>[12x]GPGSMTIIEVKIKKLENFLGNLPEYATEHSAGMDLVAANEQSITIKVGSIQLIPTGIAIALPESFEAQIRPRSGLAVKHGITVANSPGTIDADYRG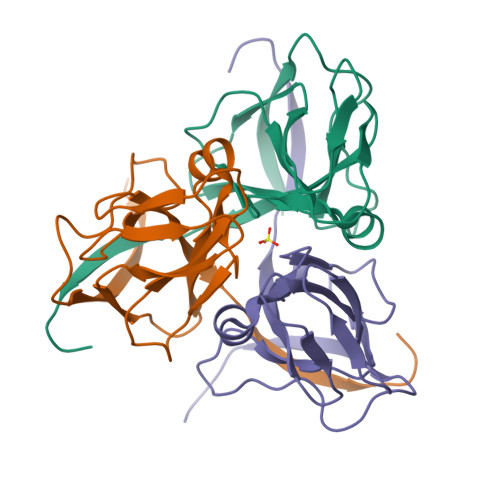EIKVLLINLGNKDFIIEKGMRIAQMIIAKYERVLWAETSILTETMRGRGGFGSTGL>AEKPKLHYFNARGRMESTRWLLAAAGVEFEEKFIKSAEDLDKLRNDGYLMFQQVPMVEIDGMKLVQTRAILNYIASKYNLYGKDIKERALIDMYIEGIADLGEMILLLPVXPPEEKDAKLALIKEKIKNRYFPAFEKVLKSHGQDYLVGNKLSRADIHLVELLYYVEELDSSLISSFPLLKALKTRISNLPTVKKFLQPGSPRKPPMDEKSLEEAR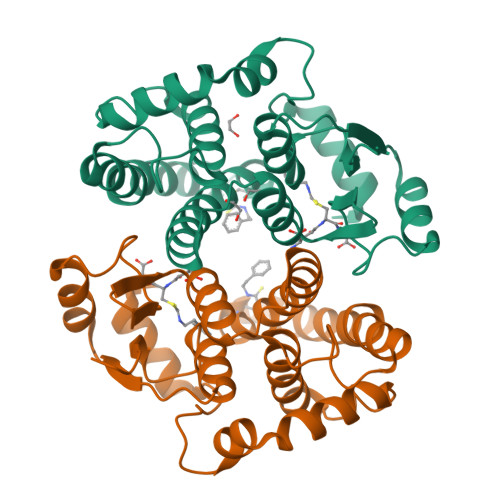KIFRF[4x]>GSHHKAVLAVRREDVNAWERRAPLAPKHIKGITNLGYKVLIQPSNRRAIHDKDYVKAGGILQEDISEACLILGVKRPPEEKLMSRKTYAFFSHTIKAQEANMGLLDEILKQEIRLIDYEKMVDHRGVRVVAFGQWAGVAGMINILHGMGLRLLALGHHTPFMHIGMAHNYRNSSQAVQAVRDAGYEISLGLMPKSIGPLTFVFTGTGNVSKGAQAIFNELPCEYVEPHELKEVSQTGDLRKVYGTVLSRHHHLVRKTDAVYDPAEYDKHPERYISRFNTDIAPYTTCLINGIYWE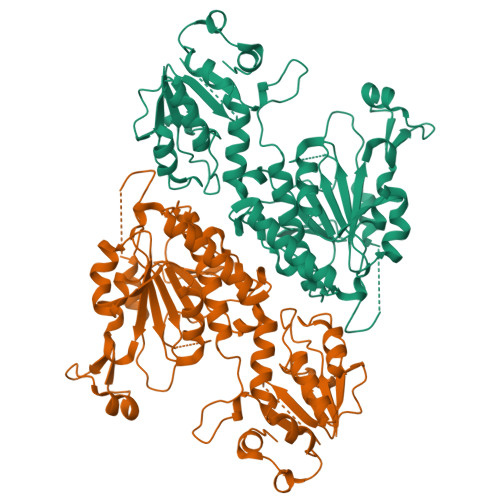QNTPRLLTRQDAQSLLAPGKFSPAGVEGCPALPHKLVAICDISADTGGSIEFMTECTTIEHPFCMYDADQHIIHDSVEGSGILMCSIDNLPAQLPIEATECFGDMLYPYVEEMILSDATQPLESQNFSPVVRDAVITSN[2x]> GPMTSQKLVRLPGLIDVHVHLREPGGTHKEDFASGTAAALAGGITMVCAMPNTRPPIIDAPALALAQKLAEAGARCDFALFLGASSENAGTLGTVAGSAAGLKLYLNETTSELRLDSVVQWMEHFETWPSHLPIVAHAEQQTVAAVLMVAQLTQRSVHICHVARKEEILLIKAAKARGLPVTCEVAPHHLFLSHDDLERLGPGKGEVRPELGSRQDVEALWENMAVIDCFASDHAPHTLEEKCGSRPPPGFPGLETMLPLLLTAVSEGRLSLDDL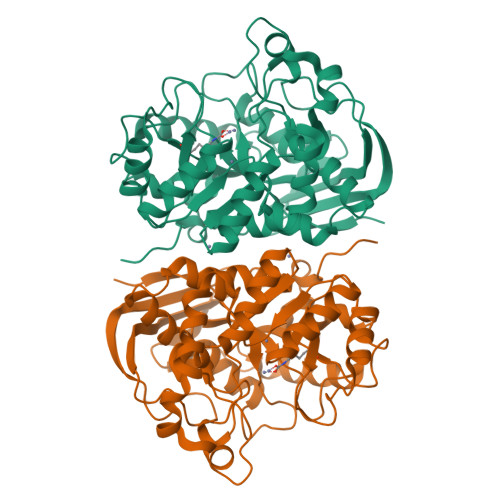LQRLHHNPRRIFHLPPQEDTYVEVDLEHEWTIPSHMPFSKAHWTPFEGQKVKGTVRRVVLRGEVAYIDGQVLVPPGYGQDVRKWPQGAVPQLPPSAPATSEMTTTPERPRRGIPGLPD> GASKGNLLSPDRILTVAHRGASGYVPEHTILSYETAQKMKADFIELDLQMTKDGKLIVMHDEKLDRTTNGMGWVKDHTLADIKKLDAGSWFNEAYPEKAKPQYVGLKVPTLEEVLDRFGKHANYYIETKSPDTYPGMEEKLIASLQKHKLLGKHSKPGQVIIQSFSKESLVKVHQLQP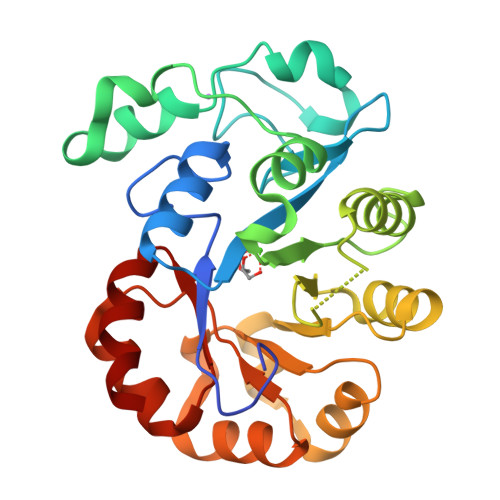NLPTVQLLEAKQMASMTDAALEEIKTYAVGAGPDYKALNQENVRMIRSHGLLLHPYTVNNEADMHRLLDWGVTGVFTNYPDLFHKVKKGY>[2x]GSGS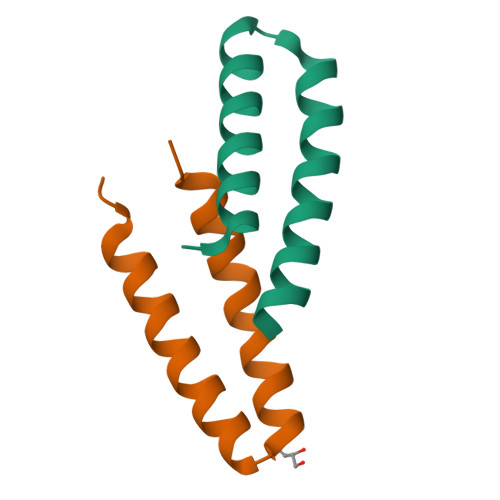PLAQQIKNIHSFIHQAKAAGRMDEVRTLQENLHQLMHEYFQQSD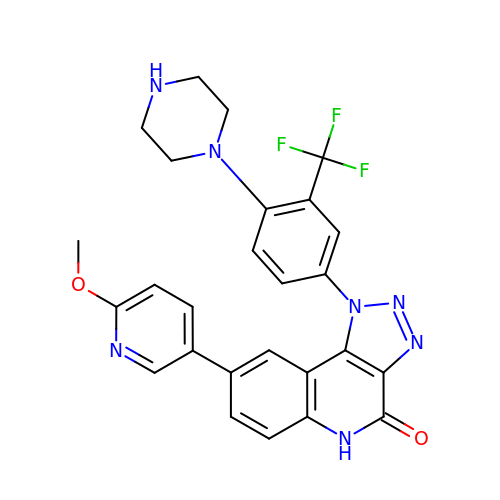8-(6-methoxypyridin-3-yl)-1-[4-piperazin-1-yl-3-(trifluoromethyl)phenyl]-5H-[1,2,3]triazolo[4,5-c]quinolin-4-one | C26 H22 F3 N7 O2 | RGHLRMNPUGUZEY-UHFFFAOYSA-N> MEVTVPDALKDRIALKKTARQLNIVYFLGSDTEPVPDYERRLSELLLYLQQFYGKEMQRHGYGARSFGLDIKSPGRVNIIEYKAKNPAAHYPYENGGGWKAAQELDEFFKAHPDRKKSQHTLIIMPTWNDEKNGPDNPGGVPFYGMGRNCFALDYPAFDIKHLGQKTREGRLLTKWYGGMAHELGHGLNLPHNHQTASDGKKYGTALMGSGNYTFGTSPTFLTPASCALLDACEVFSVTPSQQFYEGKPEVEVGDVAISFKGDQILVSGNYKSPQTVKALNVYIQDPPYAVNQDYDAVSFSRRLGKKSGKFSMKIDKKELEGLNNNEFRISLMFILANGLHMQKHFTFHWDALQDYRDGSKSGSGHHHHHH

Here we focus on OgpA from A. muciniphila, a recently discovered O-glycopeptidase that exclusively hydrolyzes the peptide bond N-terminal to serine or threonine residues substituted with an O-glycan. OgpAWT comprises two domains from the N- to the C-terminus: (i) a catalytic domain (residues 25–262) followed by (ii) a β-sandwich domain (residues 263-385). Interestingly, a Zn2+ atom coordinates with the side chains of three histidine residues, H205, H209, and H215, a highly conserved triad among metalloproteases. A glutamate residue, E206, is well-positioned to act as a general base/acid during catalysis.

The crystal structure of full-length OgpA in its unliganded form was solved using zinc single-wavelength anomalous dispersion (Zn-SAD). The high quality of the electron density maps allowed the trace of residues 27–380 (OgpAWT1) and 25 to 382 (OgpAWT2). The overall protein scaffold and the conformation of the OgpAWT1 and OgpAWT2 were essentially preserved (root mean square deviation, r.m.s.d., of 0.37 Å for 350 residues). However, the connecting loop α4–α5 (loop 9; residues 227–246) is unstructured in OgpAWT2 whereas in OgpAWT1 displays a short α-helix. Furthermore, we were unable to fully model the β7–β8 connecting loop (loop 12; residues 309–320) on OgpAWT2 crystal structure because it is disordered. A close inspection of the two crystal structures revealed that the protein crystallized as a monomer. The first β-sheet of the antiparallel β-sandwich domain consists of four β-strands with topology β6–β7–β8–β11, whereas the second β-sheet comprises four β-strands with topology β13–β12–β9–β10, with an overall size of 39 × 28 × 19 Å (“Methods” section). Both domains are separated by a long and open groove that runs parallel to the protein surface where the active site is located.> SDDRFLREKQAKLAEKIREFNDARQRGTPFYICRDLADLESKSGDRHGPHIVEAYRAVMEMVGEHPDAGEAPRERQFAKMYLDPNTQSANALAMRKQILKGATTFLEKQFWNEVNSLIAKYPQDANLGGLPDVVSKIKAYIRLRIARKTLVPDNVELQQINGEYVWAIVFYLLRAGFVTEAAQYVNSNQAHFRAIDRTFSGYINSYASSEERRLKRQMQDRCMSEYNQRIRNAPEGSIDPFRMACYKIIGRCDLSNRSLDGLQTDVNDWIWLQFNLARETDRSLELAGESYGLAELQASIREIGLKHFPKTAAEDTNGSFGMFFYLQILAGMFEQAIAYLYPFSYVDAVHFAIALTYYGLLRPVDAASAGNELLSHNTRSMPQINFGRMLGYYTRDFRAANPAAAVDYLVLICLNADEAAGGQQAQAALCHEALRELVLESREFSRLIGDIRPDGRRIRGVIEERGPLIALGQEDDFIRTITLQAASFADDNGRTTDAVLLYHLAEDYDTVVSIVSRALSEAISLEIGEDPMRLIPVKPRVTNAEGQVEEAAPGSSLSLAAIDDPVELAKAMMGMYERDHMFWQKIREPNRVACSVLLQMADIKSLVEQGRWAECLDKIRALDILPLTARGDPGTIRSYAARFPSLAQP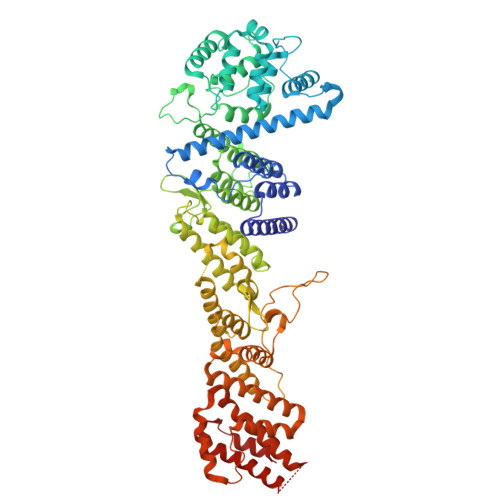VAINVPNLLMWTVLCCMRQRERLAGGQFAGNESTARLMMDELKQMTVDLMAYTSQLRYRLPPHLHEALARASAD The replicative DNA polymerase from the hyperthermophilic archaeon Pyrococcus furiosus (Pfu) is a member of that polB family and is used extensively in biotechnology applications including high-fidelity PCR. We had previously used polymerase evolution by short patch compartmentalised self-replication (spCSR) to discover variants of Pfu with a dramatically enhanced ability to incorporate Cy3- and Cy5-labelled dCTP and replicate Cy-dye labelled DNA. The resulting variant E10, derived from an exonuclease-deficient version of Pfu polymerase (with mutations V93Q, D141A and E143A) and with additional mutations in the conserved A- (V337I, E399D, N400D, R407I) and C- active site sequence motifs (Y546H) was able to efficiently PCR DNA while completely replacing all dCTP on both strands with cyanine labelled dCTP (Cy3-dCTP or Cy5-dCTP) giving rise to highly-fluorescent products, termed Cy-DNA with applications in advanced microscopy applications. In an attempt to better understand the molecular basis for the altered substrate specificity of Pfu E10 polymerase and generally gain a better structural understanding of the primer-template duplex recognition in this class of DNA polymerases, we have solved the crystal structures of the apo Pfu-E10 and a Pfu-E10:DNA binary complex at 2.4 Å and 2.9 Å resolution respectively and compare them to previously obtained structures.

Pfu-E10 polymerase was crystallised with a primer template duplex of DNA with a 2′–3′ dideoxy terminal cytosine at the 3′ end of the primer to stall the polymerase. The structure of the binary complex was solved at 2.9 Å resolution using the apo Pfu-E10 structure as the molecular replacement model. The presence of the DNA stabilises some parts of the thumb domain and density was visible for three regions that were missing in the model for the apo form (residues 612–614, 669–675 and 693–695). The density for the double stranded region of the DNA is very clear (template T4-T11 and primer P1-P8), however there is no visible density for the template base (T3) that would bind that incoming nucleotide triphosphate or for template bases T1 and T2. However, there is no evidence for a bound nucleotide triphosphate at the active site, in spite of the presence of 10 mM dCTP in the crystallisation medium. The Pfu-E10:DNA binary complex has three residues making minor-groove interactions: Tyr 495, Arg 613 and Lys 593. The largest difference involves the thumb domain, which has rotated by approximately 21 degrees from the base of the thumb to enclose the DNA and residue Leu 687 in the binary complex has moved 18 Å from its position in the apo form. In the RB6 structure the fingers domain closes inwards towards the dNTP, whereas in the Pfu-E10:DNA binary complex the fingers domain remains in the orientation observed in the structure of the apo enzyme, consistent with the absence of a bound dNTP at the active site.

> MILDVDYITEEGKPVIRLFKKENGKFKIEHDRTFRPYIYALLRDDSKIEEVKKITGERHGKIVRIVDVEKVEKKFLGKPITVWKLYLEHPQDQPTIREKVREHPAVVDIFEYDIPFAKRYLIDKGLIPMEGEEELKILAFAIATLYHEGEEFGKGPIIMISYADENEAKVITWKNIDLPYVEVVSSEREMIKRFLRIIREKDPDIIVTYNGDSFDFPYLAKRAEKLGIKLTIGRDGSEPKMQRIGDMTAVEVKGRIHFDLYHVITRTINLPTYTLEAVYEAIFGKPKEKVYADEIAKAWESGENLERVAKYSMEDAKATYELGKEFLPMEIQLSRLIGQPLWDVSRSSTGNLVEWFLLRKAYERNEVAPNKPSEEEYQRRLRESYTGGFVKEPEKGLWDDIVYLDFIALYPSIIITHNVSPDTLNLEGCKNYDIAPQVGHKFCKDIPGFIPSLLGHLLEERQKIKTKMKETQDPIEKILLDYRQKAIKLLANSFYGYYGYAKARWYCKECAESVTAWGRKYIELVWKELEEKFGFKVLYIDTDGLHATIPGGESEEIKKKALEFVKYINSKLPGLLELEYEGFYKRGFFVTKKRYAVIDEEGKVITRGLEIVRRDWSEIAKETQARVLETILKHGDVEEAVRIVKEVIQKLANYEIPPEKLAIYEQITRPLHEYKAIGPHVAVAKKLAAKGVKIKPGMVIGYIVLRGDGPISNRAILAEEYDPKKHKYDAEYYIENQVLPAVLRILEGFGYRKEDLRYQKTRQVGLTSWLNIKKS N-[(1R,3R)-3-hydroxy-1-(hydroxymethyl)-3-phenylpropyl]tridecanamide 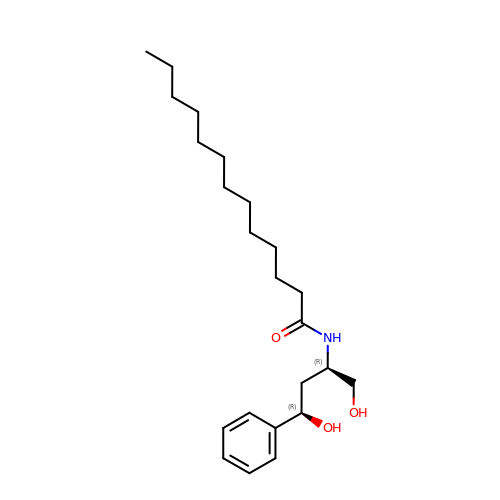| C23 H39 N O3 | QFIYNRCZMOYKEJ-FGZHOGPDSA-N> GA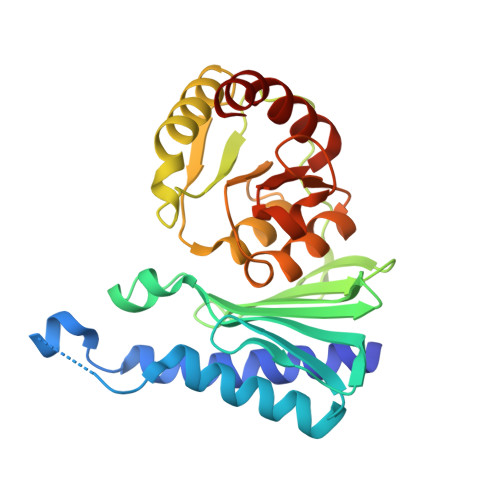MAMHPMLNIAVRAARKAGNLIAKNYETPDAVEASQKGSNDFVTNVDKAAEAVIIDTIRKSYPQHTIITEESGELEGTDQDVQWVIDPLDGTTNFIKRLPHFAVSIAVRIKGRTEVAVVYDPMRNELFTATRGQGAQLNGYRLRGSTARDLDGTILATGFPFKAKQYATTYINIVGKLFNECADFRRTGSAALDLAYVAAGRVDGFFEIGLRPWDFAAGELLVREAGGIVSDFTGGHNYMLTGNIVAGNPRVVKAMLANMRDELSDALKR> SENTFLHPIIQIDRSFM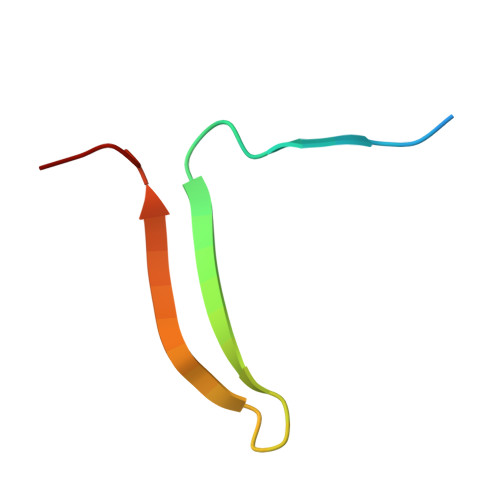LLILERSTRSILFLGKVVNPTEA> GAMAGKKVLIVYAHQEPKSFNGSLKNVAVDELSRQGCTVTVSDLYAMNFEPRATDKDITGTLSNPEVFNYGVETHEAYKQRSLASDITDEQKKVREADLVIFQFPLYWFSVPAILKGWMDRVLCQGFAFDIPGFYDSGLLQGKLALLSVTTGGTAEMYTKTGVNGDSRYFLWPLQHGTLHFCGFKVLAPQISFAPEIASEEERKGMVAAWSQRLQTIWKEEPIPCTAHWHFGQ

NQO2 is a cytosolic flavoprotein that carries out the 2-electron reduction of quinones using electron donors such as nicotinamide riboside (NRH). It is one of two closely related cellular quinone reductases (the other being NQO1) and is thought to be involved in metabolic reduction and xenobiotic detoxification, although its precise physiological role remains uncertain. Biochemical and structural studies have demonstrated that NQO2 is a dimer. Dimerization leads to formation of two FAD-containing active sites per dimer, with each active site located in a deep pocket at the interface between monomers.

We have solved the X-ray crystal structure of NQO2 bound to imatinib to 1.75 Å resolution, which shows that the drug is bound adjacent to the flavin isoalloxazine ring. The complex crystallized in space group I422, with one monomer in the asymmetric unit. The final model includes residues 3–230 of human NQO2, one FAD molecule, one imatinib molecule, one zinc atom, two (4R)-2-methylpentane-2,4-diol (MRD) molecules, and 213 solvent molecules. In our structure, the dimer is formed from two adjacent molecules related by a crystallographic 2-fold axis. The isoalloxazine ring of the flavin cofactor forms the floor of the active site, upon which the pyridine and pyrimidine rings (rings A and B) of the bound imatinib stack, with an average distance of ~3.3 Å between atoms in closest contact. The side chains of Trp 105 and Phe 106 form the back of the active site, while three hydrophobic amino acids from the other monomer in the NQO2 dimer, Phe 126, Ile 128, and Phe 178, form the top of the active site. Steric constraints prevent the bound imatinib from binding in an extended conformation, causing it to instead adopt a horseshoe shape that directs the methylbenzene, benzamide, and N-methylpiperazine rings (rings C, D and E) away from the active site and towards the solvent. The inhibitor makes no direct hydrogen bonds with the protein, although several water-mediated hydrogen bonds are observed. A water-mediated hydrogen bond is formed between Asn 161, which is positioned by a hydrogen-bonding interaction with Tyr 132, and the N3 nitrogen of the imatinib pyridine ring (ring A). The conformation of the imatinib molecule in complex with NQO2 resembles this cis conformation.2-OXALOSUCCINIC ACID | C6 H6 O7 | 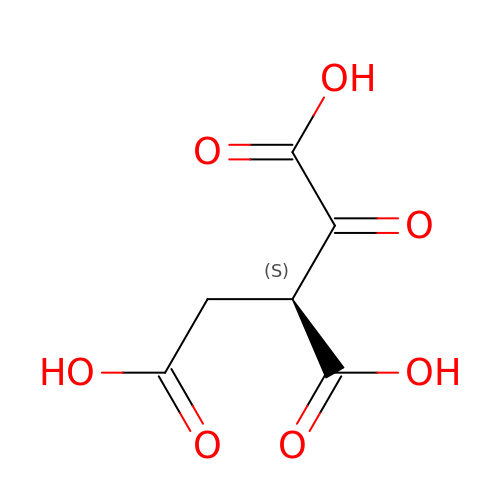UFSCUAXLTRFIDC-REOHCLBHSA-N>[3x]MDTKGRLVAGSHNRNEFVLINADETARVAVTELSGQICQICGDELEVTVNGEPFVACNECAFPVCRPCYEYERREGNQVCPQCKTRYKRIKGSPRVEGDEEEDDSDDLESEFDIGSVFSARLNYGSQVNGSVIHAPSEFDAASVASEIPLLTYGQEDVGISADKHALILPPFTARGKRVHPMPFPDSSVPVQPRPMDPKKDIAVYGYGSVAWKERMEDWKKKQSEKLQVVRHEGGKDSDELDDPDLPKMDEGRQPLWRKLPISSSRINPYRIIIVLRIAILCLFFHYRILHPVNDAYALWLTSVICEIWFAVSWIFDQFPKWSPILRETYLDRLSLRYEKEGKPSLLADIDVFVSTVDPMKEPPLITANTVLSILAVDYPVDKVACYVSDDGAAMLTFEALSETSEFARKWVPFCKKFCIEPRAPEWYFAQKVDYLKDKVDATFIRERRAIKREYEEFKVRINALVALAQKVPEDGWTMQDGTPWPGNNVRDHPGMIQVFLGQNGVRDIEGNELPRLVYVSREKRPGYDHHKKAGAMNALVRVSAIITNAPYVLNVDCDHYINNSKALREAMCFMMDPTSGKKICYVQFPQRFDGIDRHDRYSNRNVVFFDINMKGLDGIQGPIYVGTGCVFRRQAFYGYDAPTSKKAPRKTCNCWPKWCCCLCCGSKKKKIKAKSSVKKKIKNKDDIKQMHALENIEEGIEGIDNEKSSLMSQSKFEKKFGQSSVFIASTLLEDGGVPKAASSATLLKEAIHVISCGYEDKTEWGKEVGWIYGSVTEDILTGFKMHCHGWRSVYCMPKRPAFKGSAPINLSDRLHQVLRWALGSVEIFFSRHCPIWYGYGGGLKSLERFSYINSVVYPLTSIPLIAYCALPAVCLLTGKFIVPEISNYASIIFMALFISIAATGILEMQWGGVGIHDWWRNEQFWVIGGASSHLFALFQGLLKVLAGVNTNFTVTSKAADDGEFADLYIFKWTSLLIPPLTLLIINIIGVIVGVSDAINNGYDSWGPLFGRLFFALWVIVHLYPFLKGVMGKQEGVPTIILVWAILLSSILTLLWVRINPFLAKSDVVLEICGLNCD

Cellulose is synthesized by cellulose synthase (CesA), a membrane-integrated processive family-2 glycosyltransferase (GT; Lombard et al., 2014). The enzyme synthesizes cellulose from UDP-activated glucose (UDP-Glc) and translocates the polymer across the plasma membrane through a channel formed by its own membrane-spanning segment. While bacterial CesAs primarily function as monomeric enzymes, structural analyses of plant CesAs revealed their assembly into triangular-shaped trimeric complexes of three catalytically active subunits. Cryo-EM analyses of all three CesA isoforms reveal the formation of homotrimeric complexes, similar to the secondary cell wall CesAs.

Of note, compared to GmCesA1 and GmCesA3, the yield of trimeric GmCesA6 was more variable, with some preparations producing primarily monomeric species. This suggests that GmCesA6 is less stable in a detergent-solubilized state compared with the other isoforms. The helix has been modeled for GmCesA1 and GmCesA6, while its density is detectable at a similar position but too discontinuous for modeling in the GmCesA3 map. The displacement of TM helix 7 away from the TM channel of the neighboring subunit opens a lateral lipid-exposed window in the neighboring subunit’s channel architecture. About midway across the membrane, the opening is roughly 6 Å wide, for example between the side chains of Ile901 in TM helix 4 and Trp1018 in TM helix 6. The triangular PCR arrangement in a CesA complex positions the side chains of conserved Lys and Arg residues towards the threefold symmetry axis. These residues include Arg449, Lys452, and Arg453 in GmCesA6 and coordinate unidentified ligand(s) on the membrane distal and proximal side of the PCR triangle. Inactivation could be due to modification of a conserved cysteine residue in CesA’s catalytic pocket (such as Cys558 or Cys630 in GmCesA6). In contrast, the activities of GmCesA1 and GmCesA6 peak at pH 8, with a slight decline at pH 9. GmCesA1’s apparent IC50 for UDP is about 0.8 mM, whereas this concentration is increased to about 1.3–1.5 mM for GmCesA6 and GmCesA3, respectively.> GSQKERLLDELTLEGVARYMQSERCRRVICLVGAGISTSAGIPDFRSPSTGLYDNLEKYHLPYPEAIFEISYFKKHPEPFFALAKELYPGQFKPTICHYFMRLLKDKGLLLRCY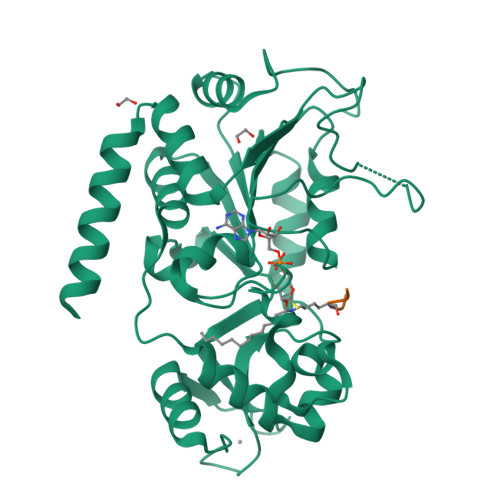TQNIDTLERIAGLEQEDLVEAHGTFYTSHCVSASCRHEYPLSWMKEKIFSEVTPKCEDCQSLVKPDIVFFGESLPARFFSCMQSDFLKVDLLLVMGTSLQVQPFASLISKAPLSTPRLLINKEKAGQSDPFLGMIMGLGGGMDFDSKKAYRDVAWLGECDQGCLALAELLGWKKELEDLVRREHASIDAQ;> PKKTG> MAQVINTNSLSLLTQNNLNKSQSALGTAIERLSSGLRINSAKDDAAGQAIANRFTANIKGLTQASRNANDGISIAQTTEGALNEINNNLQRVRELAVQSANSTNSQSDLDSIQAEITQRLNEIDRVSGQTQFNGVKVLAQDNTLTIQVGANDGETIDIDLKQINSQTLGLDTLNVQQKYKVSDTAATVTGYADTTIALDNSTFKASATGLGGTDQKIDGDLKFDDTTGKYYAKVTVTGGTGKDGYYEVSVDKTNGEVTLAGGATSPLTGGLPATATEDVKNVQVANADLTEAKAALTAAG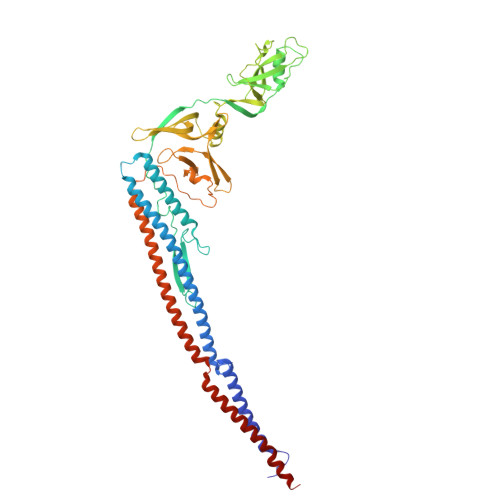VTGTASVVKMSYTDNNGKTIDGGLAVKVGDDYYSATQNKDGSISINTTKYTADDGTSKTALNKLGGADGKTEVVSIGGKTYAASKAEGHNFKAQPDLAEAAATTTENPLQKIDAALAQVDTLRSDLGAVQNRFNSAITNLGNTVNNLTSARSRIEDSDYATEVSNMSRAQILQQAGTSVLAQANQVPQNVLSLLR> MTQELGNANFENFIGATEGFSEIAYQFTSHILTLGYAVMLAGLLYFILTIKNVDKKFQMSNILSAVVMVSAFLLLYAQAQNWTSSFTFNEEVGRYFLDPSGDLFNNGYRYLNWLIDVPMLLFQILFVVSLTTSKFSSVRNQFWFSGAMMIITG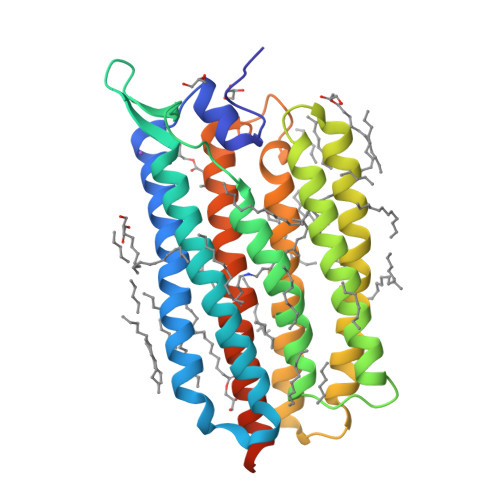YIGQFYEVSNLTAFLVWGAISSAFFFHILWVMKKVINEGKEGISPAGQKILSNIWILFLISWTLYPGAYLMPYLTGVDGFLYSEDGVMARQLVYTIADVSSKVIYGVLLFNLAITLSKNKELVEANSLEHHHHHH1-[cis-4-(3-methylphenyl)cyclohexyl]-4-(pyridin-3-yl)piperazine | C22 H29 N3 | 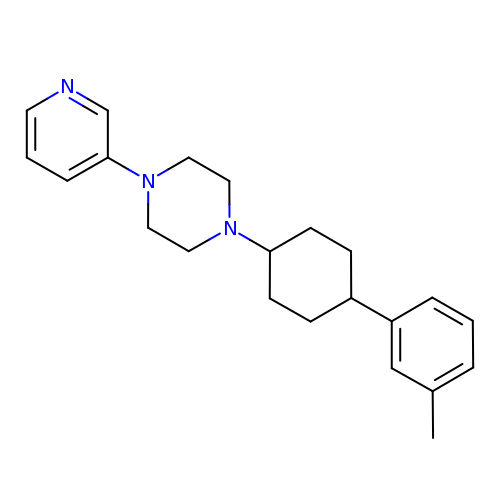QANXJBIOBLNORO-TYKWCNGQSA-N>AYSNTYQEFTNIDQAKAWGNAQYKKYGLSKSEKEAIVSYTKSASEINGKLRQNKGVINGFPSNLIKQVELLDKSFNKMKTPENIMLFRGDDPAYLGTEFQNTLLNSNGTINKTAFEKAKAKFLNKDRLEYGYISTSLMNVSAFAGRPIITKFKVAKG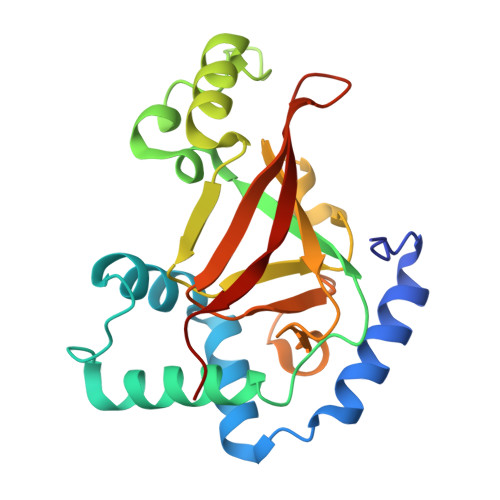SKAGYIDPISAFAGQLEMLLPRHSTYHIDDMRLSSDGKQIIITATMMGTAINPK[4x]>SIIRPQLKFREKIDNSNTPFLPKIFIKPNAQKPLPQALSKERRERPQDRPEDLDVPPALADFIHQQRTQQVEQDMFAHPYQYELNHFTPADAVLQKPQPQLYRPIEETPCHFISSLDELVELNEKLLNCQEFAVNLEHHSYRSFLGLTCLMQISTRTEDFIIDTLELRSDMYILNESLTDPAIVKVFHGADSDIEWLQKDFGLYVVNMFDTHQAARLLNLGRHSLDHLLKLYCNVDSNKQYQLADWRIRPLPEEMLSYARDDTHYLLYIYDKMRLEMWERGNGQPVQLQVVWQRSRDIC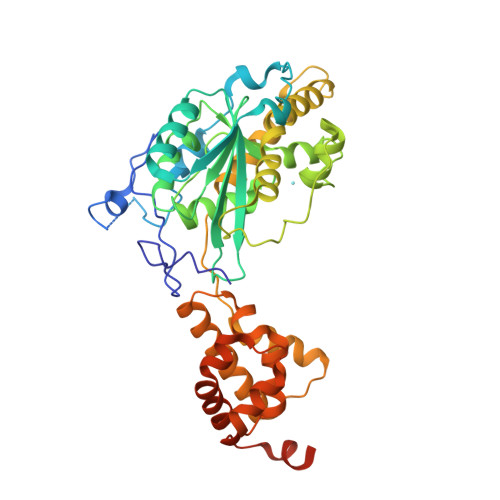LKKFIKPIFTDESYLELYRKQKKHLNTQQLTAFQLLFAWRDKTARREDESYGYVLPNHMMLKIAEELPKEPQGIIACCNPVPPLVRQQINEMHLLIQQAREMPLLKSEVAAGVKKSGPLPSAERLENVL[2x]However, the development of endolysins as mainstream antibacterial agents first requires a comprehensive biochemical understanding. This study defines the atomic structure and enzymatic function of Escherichia coli O157:H7 phage FAHEc1 endolysin, LysF1. BLASTp analysis with non-redundant protein sequences indicated that LysF1 belongs to the lysozyme-like glycoside hydrolase family 24 (GH24). This group contains phage endolysins, such as the well-studied T4 lysozyme (T4L), and bacterial autolysins, which cleave the β-1,4 glycosidic bond between N-acetylmuramic acid and N-acetylglucosamine in peptidoglycan. The multisequence alignment reveals that LysF1 contains these conserved residues with Glu15, Asp24 and Thr30.

To better understand the mechanism by which LysF1 functions, we crystallized LysF1 and solved the structure to a maximum resolution of 1.71 Å. The structure contains two protein molecules in the asymmetric unit each comprising the full endolysin sequence derived from FAHEc1 (residues 1–154) and two phosphates. The completed model reveals that the overall architecture of LysF1 consists of three regions, a catalytic loop region (Glu15–Lys41), a connector helix (α2, Ala51–Lys71) and a C-terminal α-helix bundle (α3–α7, Gln79–Asp149). The protein exhibits a cleft between the catalytic loop region and the α-helix bundle where peptidoglycan is proposed to bind. The catalytic loop region contains a β-hairpin (β1–β2), a structural element that is conserved across the glycoside hydrolase lysozyme super family and contains predicted catalytic residues Asp24 and Thr30. A putative catalytic residue Glu15 is positioned at the C-terminal end of α1 facing into the cleft. The catalytic residues of LysF1 are positioned 8.9 Å apart, consistent with T4L-like endolysins, which would accommodate the peptidoglycan and water molecule between the side chains for catalysis. Therefore, the catalytic site of LysF1 is consistent with a peptidoglycan hydrolase that inverts the anomeric center of the peptidoglycan glycoside during catalysis. Inspection of the LysF1 crystal structure revealed the unusual appearance of a charged side chain (from Glu88) positioned within the hydrophobic core of the α-helix bundle. Wild type LysF1 had a melting temperature of 53.6 °C. Glu88Leu was the most stabilizing mutation, increasing the melting temperature by 9.4 °C. The methionine and phenylalanine mutations increased stability by 7.1 °C and 4.0 °C, respectively.

>LYFQGHMQLSRKGLDAIKFFEGLELEAYEDSAGIPTIGYGTIRIDGKPVKMGMKITAEQAEQYLLADVEKFVAAVNKAIKVPTTQNEFDALVSETYNIGITAMQDSTFIKRHNAGNKVGCAEAMQWWNKVTVKGKKVTSNGLKNRRRMEADIYLDSVYPK[2x]> CELDRDPEGKDFQQPYTSFVQTKQNRDGLYALLRNTENPRMHFYQELQSDMYCTTITDGNSLAPFVNWDLGILNDHGRADEDEVSGIAGYYFV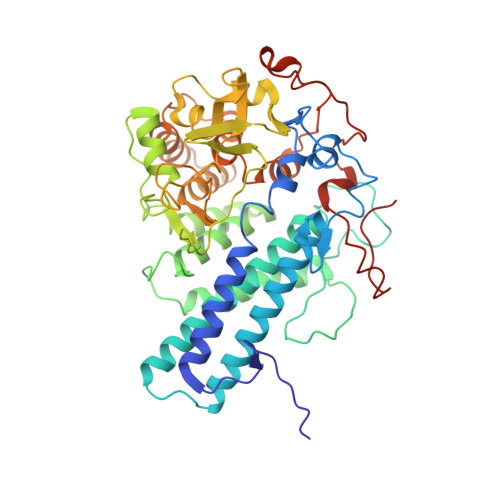YNRLNQQANAFVNNTEAALQNQVYKNSTEIANAKSFLAEGKVLQALAIWRLMDRFSFHESVTEVNSGAKDLGVILLKEYNPGYIGPRATKAQCYDYILSRLSEAIEVLPENRESVLYVSRDYAYALRARIYLALGEYGKAAADAKMVVDKYPLIGAADASEFENIYRSDANNPEIIFRGFASATLGSFTATTLNGAAPAGKDIKYNPSAVPFQWVVDLYENEDFRKSVYIAKVVKKDKGYLVNKFLEDKAYRDVQDKPNLKVGARYFSVAEVYLILVESALQTGDTPTAEKYLKALSKARGAEVSVVNMEALQAERTRELIGEGSRLRDMVRWSIPNNHDAFETQPGLEGFANTTPLKAQAPVGFYAYTWEFPQRDRQTNPQLIKNWPI> GEVNKIIGSRTAGEGAMEYLIEWKDGHSPSWVPSSYIAADVVSEYETPWWTAARKADEQALSQLLEDRDVDAVDENGRTALLFVAGLGSDKCVRLLAEAG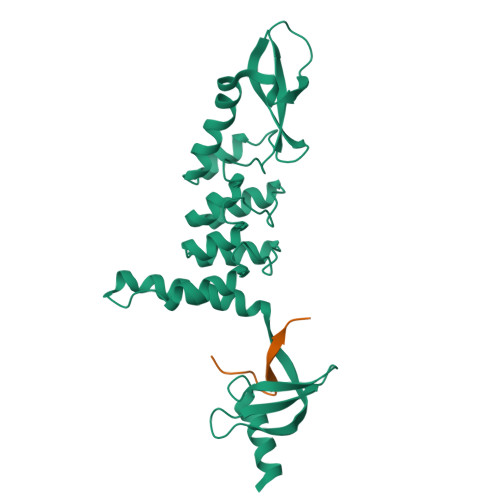ADLDHRDMRGGLTALHMAAGYVRPEVVEALVELGADIEVEDERGLTALELAREILKTTPKGNPMQFGRRIGLEKVINVLEGQVFEYAEVDEIVEKRGKGKDVEYLVRWKDGGDCEWVKGVHVAEDVAKDYEDGLEYAVAESVIG;> QKAPPGTARRKRK>MVSAIVLYVLLAAAAHSAFAAMVHHHHHHSAEETLMDSTTATAELGWMVHPPSGWEEVSGYDENMNTIRTYQVCNVFESSQNNWLRTKFIRRRGAHRIHVEMKFSVRDCSSIPSVPGSCKETFNLYYYEADFDSATKTFPNWMENPWVKVDTIAADESFSQVDLGGRVMKINTEVRSFGPVSRSGFYLAFQDYGGCMSLIAVRVFYRK[2x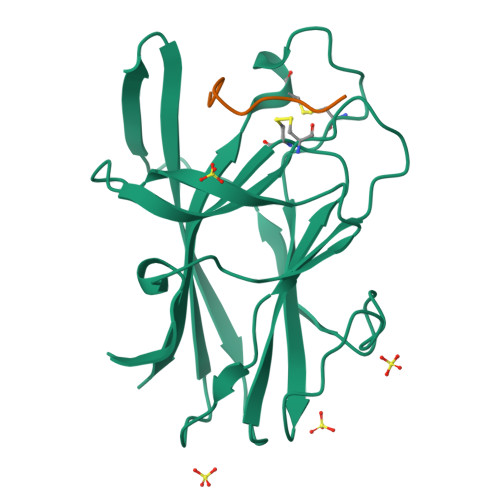];>SNEWIQPRLPQH[2x]>MLVKGNEILLKAHKEGYGVGAFNFVNFEMLNAIFEAGNEENSPLFIQASEGAIKYMGIDMAVGMVKIMCERYPHIPVALHLDHGTTFESCEKAV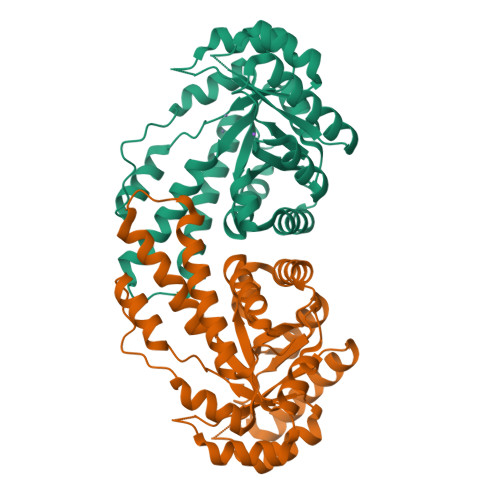KAGFTSVMIDASHHAFEENLELTSKVVKMAHNAGVSVEAELGRLMGIEDNISVDEKDAVLVNPKEAEQFVKESQVDYLAPAIGTSQGAFKFKGEPKLDFERLQEVKRLTNIPLVLHGASAIPDNVRKSYLDAGGDLKGSKGVPFEFLQESVKGGINKVNTDTDLRIAFIAEVRKVANEDKSQFDLRKFFSPAQLALKNVVKERMKLLGSANKI[2x]Laccases, also classified as benzenediol/oxygen oxidoreductases with an Enzyme Commission (EC) number of 1.10.3.2, are multi-copper oxidases having 4 copper atoms arranged with oxygen at its center. The 4 copper atoms are termed Cu T1 (where the reducing substrate binds) and trinuclear copper cluster T2/T3. Laccases have been shown to catalyze the oxidation of phenols, polyphenols, and non-phenolic aromatic compounds through a free radical mechanism, where the enzyme facilitates the transfer of electrons from the substrates to molecular oxygen, resulting in the formation of water and oxidized products. In this work, we present the crystal structure of a CotA-laccase enzyme derived from Bacillus licheniformis ATCC 9945a (referred to in this paper as Bli-Lacc) adding to the growing database of CotA-laccases.

The current model at 2.7 Å resolution has an Rmodel of ~17% and an Rfree of ~23%. The model consisted of residues 2–509 and therefore the residues beyond 513 that were added during cloning were not visible in the density. As found in several other laccase structures, two loops were disordered hence not interpreted with an atomic model: residues 90–96 and 359–361. The root mean square deviation (RMSD) between the two structures was 0.5 Å sharing 66% sequence identity and 78% similarity. Notably, two loops, 213–219 and 319–327, are immediately adjacent to the substrate binding site. Aside from the disordered region at 356–362, the most flexible is the 213–218 loop adjacent to the substrate binding pocket. Therefore, the most divergent and conformationally flexible regions appear to be involved with substrate selectivity and affinity. As expected, the most highly conserved residues are those in the vicinity of the bound metals and/or those in the core of the protein. To further validate and confirm the resemblance of the Bli-Lacc against other laccases with solved crystal structures, a multiple sequence alignment using the amino acid sequences was executed and motifs characteristic of laccases were found conserved—HXHG, HXH, HXXHXH, and HCHXXXHXXXXM/L/F as can be seen in Figure 5.

>[2x]MKLEKFVDKLPIPKVLKPHSKSKEMTYYEVTMKEFQQQLHRDLPPTRLFGYNGVYPGPTFEVQKHEKVAVKWLNKLPDHHFLPVDHTIHDDGHHEHEVKTVVHLHGGRTPPDSDGYPEAWYTKDFQVKGPFFEREVYEYPNEQDATALWYHDHAMAITRLNVYAGLVGLYFIRDREERSLNLPKGEYEIPLLIQDKSFHEDGSLFYPRQPDNPSPDLPDPSIVPAFCGDTILVNGKVWPYDELEPRKYRFRILNASNTRIFELYFDHDITFHQIGTDGGLLQHPVKVNELVIAPAERCDIIVDFSRAEGKTVTLKNRIGCSGQDADPDTDANIMQFRISKPLKQKDTSSLPRILRKRPFYRRHKINTLRNLSLGASLDQYGRPVLLLNNTKWHEPVTETPALGSTEIWSIINAGRAIHPIHLHLVQFLILDHRPFDIERYQENGELVFTGPAAPPAQNEKGLKDTVKVPPGSVTRIIATFAPYSGRYVWHCHILEHEDYDMMRPLEVTDIRHQEFEAWARTKTHLRRGSE>MHKATYKERAATHPSPVAAKLFNIMHEKQTNLCASLDVRTTKELLELVEALGPKICLLKTHVDILTDFSMEGTVKPLKALSAKYNFLLFEDRKFADIGNTVKLQYSAGVYRIAEWADITNAHGVVGPGIVSGLKQAAEEVTKEPRGLLMLAELSCKG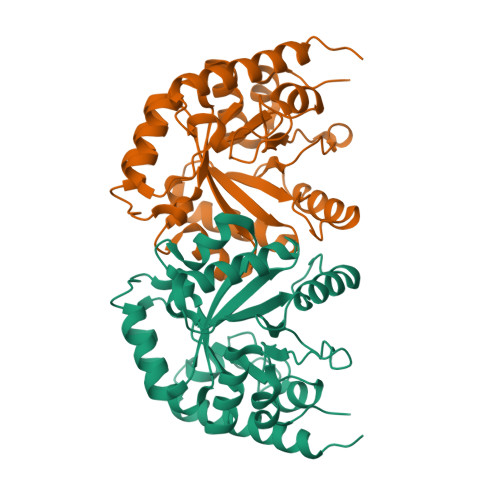SLSTGEYTKGTVDIAKSDKDFVIGFIAQRDMGGRDEGYDWLIMTPGVGLDDKGDALGQQYRTVDDVVSTGSDIIIVGRGLFAKGRDAKVEGERYRKAGWEAYLRRCGQQD[4x]>VETIELKRGSNSVYVQYDDIMFFESSTKSHRLIAHLDNRQIEFYGNLKELSQLDDRFFRCHNSFVVNRHNIESIDSKERIVYFKNKEHCYASVRN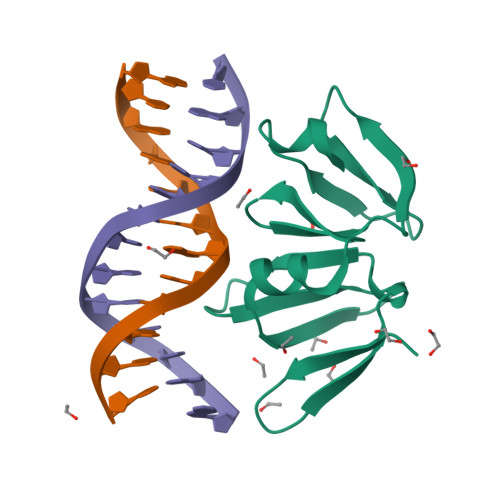VKKI[2x]> GGGQHIAIVGCVHGKYREMYRQLSEYEKSTGKEISFVICTGDMQTL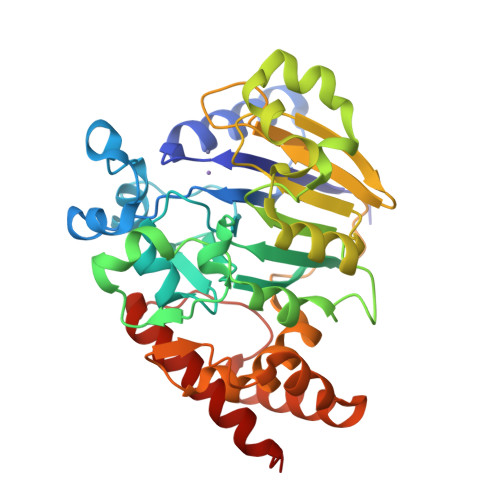RYEADLVYLKVPPKYKQMGDFHLYYEGKEKAPYLTLFIGGNHESSNVLLHLYNGGFVCFNMYYLGVCSCININGLRIVGVSGIYKSFDEKKPYTYPPSPNDVVSLFHTRNYVIQMLSNLSQSSQIDISLSHDWPQGIVMKGNYKQLYRFQPGFKKDGASLGSPINKVILNTLKPKYWISGHMHCEYHAEEGPTHFIALGKIGYKNAISYLDLPLKQKTDLEYDKDWVCNLIMTWPAFSNKAQFPDLSYSISELLSKRTKELDKKIIELWEKYIGLKIIYDSDTFDIQFTSRRFYIEKIYNELNIN>[4x]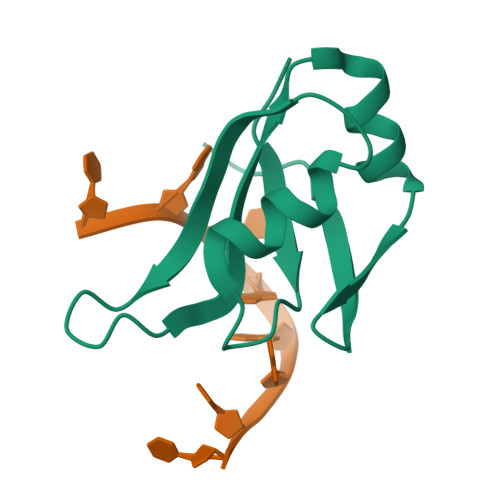MRGSHHHHHHGSQKTSDLIVLGLPWKTTEQDLKEYFSTFGEVLMVQVKKDLKTGHSKGFGFVRFTEYETQVKVMSQRHMIGGRWCDCKLPNSKQSQDEPLRSR>[2x]GAMEGFKANLSLLRRPGEKTYTQRCRLFVGNLPADITEDEFKRLFAKYGEPGEVFINKGKGFGFIKLESRALAEIAKAELDDTPMRGRQLRVRFAT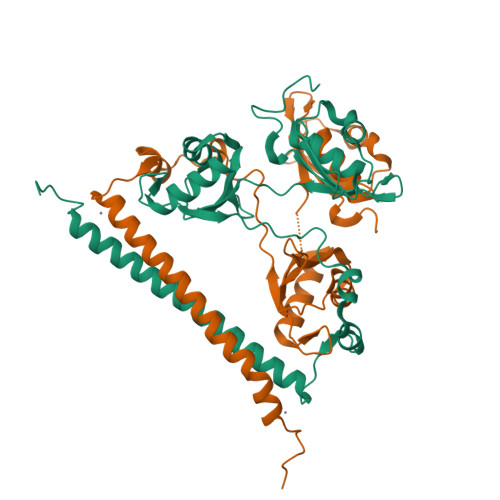HAAALSVRNLSPYVSNELLEEAFSQFGPIERAVVIVDDRGRSTGKGIVEFASKPAARKAFERCSEGVFLLTTTPRPVIVEPLEQLDDEDGLPEKLAQKNPMYQKERETPPRFAQHGTFEYEYSQRWKSLDEMEKQQREQVEKNMKDAKDKLESEMEDAYHEHQANIL As a large family of membrane proteins crucial for bacterial physiology and virulence, the Multiple Peptide Resistance Factors (MprFs) utilize two separate domains to synthesize and translocate aminoacyl phospholipids to the outer leaflets of bacterial membranes. The function of MprFs enables Staphylococcus aureus and other pathogenic bacteria to acquire resistance to daptomycin and cationic antimicrobial peptides. Here we present cryo-electron microscopy structures of MprF homodimer from Rhizobium tropici (RtMprF) at two different states in complex with lysyl-phosphatidylglycerol (LysPG). RtMprF contains a membrane-embedded lipid-flippase domain with two deep cavities opening toward the inner and outer leaflets of the membrane respectively.

The cryo-EM map of RtMprF(GDN)-nanodiscs exhibits well-defined features allowing construction of a structural model with ∼94.4% amino acid residues of the full-length RtMprF protein and identification of four lipid molecules per monomer. Strikingly, one LysPG molecule each (LysPG1 and LysPG2) is trapped in Cavities C and P of the RtMprF(GDN)-nanodisc structure. The LysPG1 molecule in Cavity C has the characteristic hook-shaped polar head group inserted deeply toward the center of Subdomain 1, while the hydrophobic fatty-acyl chains of LysPG1 extend outwardly to the inner leaflet of lipid bilayer. Unlike LysPG1, LysPG2 located in Cavity P has an extended conformation. Its head group is positioned on the periplasmic surface and both fatty-acyl chains extend deep into the cavity toward the center of Subdomain 1. The backbone glycerol-3-phosphate group of LysPG2 may bind to adjacent residues through hydrogen bonds, whereas the fatty-acyl chains form van der Waals and hydrophobic interactions with nearby residues including Arg304, Phe276, and several other hydrophobic residues. Such a well-resolved lipid feature found in Cavity P is only present in RtMprF(GDN)-nanodisc but not in RtMprF(DDM)-nanodisc. By superposing them, it is apparent that TM12 moves 2.2 Å closer to TM11 and TM14 moves 4.2 Å closer to TM9 upon binding of LysPG2 in Cavity P. Besides, the amino acid residues involved in binding the fatty-acyl chains of LysPG2 are also adjusted slightly. In comparison, the LysPG:protein stoichiometry of the RtMprF(GDN) sample is ∼2.6, much higher than the LysPG:protein stoichiometry of the RtMprF(DDM) sample. Such difference may account for the strong phospholipid density in Cavity P of RtMprF(GDN)-nanodisc due to higher occupancy of LysPG, consistent with the interpretation of the lipid as LysPG2. A second molecule of LysPG may further enter Cavity C, so that Cavities C and P are both loaded with LysPG as observed in the RtMprF(GDN)-nanodisc structure (State 5).

>[2x]MSSPIDLESADEELEERGGIVGLLNRYRALIVAVLTVAVFCIAAYAIYDLTTEVRYDDVVHALTTTKISSVLLALLFTGLSFASLIFYDQNALEYIGKRLPFPHVALTSFSAYAVGNTAGFGALSAGAIRYRAYTRLGLSPDDITRVIAFVTLAFGLGLASVGAMALLVIADEIGPLISVDGLWLRLIAIAILAALAFVVYAGRNGREVRIGPVAVRLPDSRTWSRQFLVTAFDIAASASVLYVLLPETSIGWPGFFAIYAIAVGLGVLSHVPAGFGVFETIIIAWLGSSVNEDAVLSSLVLYRVIYNVIPLVIAIAAISVAELRRFVDHPVASSMRRIGARLMPQLLSAFALLLGMMLVFSSVTPTPDHNLIVLSDYLPLSLVESAHFLSSLLGLAIIVAARGLSQRLDGAWWVSTFSALFALFFSLLKAIAIVEAGLLAFFVFSLVVSRRLFKRPASLLNQTLTAGWLTAIAVVCIGAIVVLFFVYRDVGYSNELWWQFEFADEAPRGLRAALGISIVSSAIAIFSLLRPATKRPEPVSDDAVARAVEIVRKQGVADANLVRMGDKSIMFSEKGDAFIMYGKQGRSWIALFDPVGPRQALPDLIWRFVETARAAGCRSVFYQISPALLSYCADAGLRAFKLGELAVVNLANFELKGGKWANLRQTASRAVRDGLEFAVIEPQDIPDVLDQLAHVSDTWLADHNAKEKSFSLGAFDPDYVCSQPVGVLKKDGKIVAFANILMTETKEEGSVDLMRFSPDAPKGSMDFLFVQILEYLKGEGFQRFNLGMAPLSGMSRRESAPVWDRVGGTVFEHGERFYNFKGLRAFKSKFHPEWQPRYLAVSGGVSPMIALMDATFLIGGGLKGVVRKKLAAALEHHHHHH> KKAS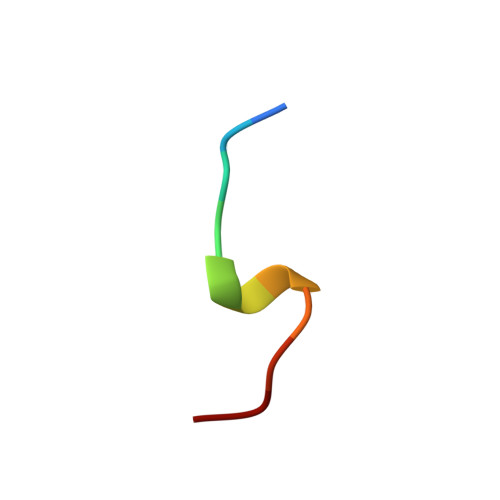LFDMFDF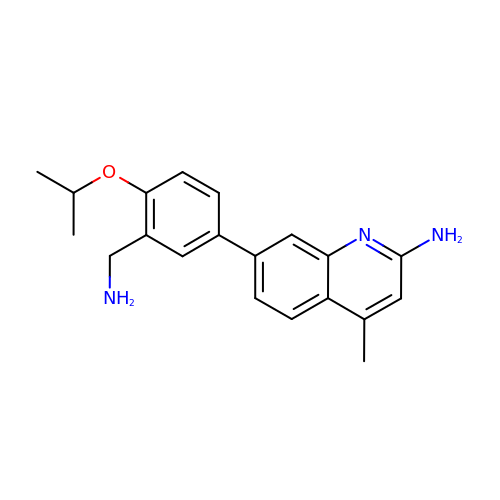7-{3-(aminomethyl)-4-[(propan-2-yl)oxy]phenyl}-4-methylquinolin-2-amine | C20 H23 N3 O | RMUSFJBGBOTWMV-UHFFFAOYSA-N The Ton and Tol systems are sophisticated molecular machineries essential for virulence and survival of Gram-negative bacteria. Both systems rely on the proton gradient at the inner membrane to produce force and movement that are transmitted to target proteins associated with the outer membrane. Ton is involved in the uptake of essential nutrients such as siderophore-iron, vitamin B12 and carbohydrates, while Tol maintains outer membrane integrity and plays an active role in cell division. We have solved the high-resolution structures of the E. coli TonB-ExbB-ExbD and TolA-TolQ-TolR complexes, revealing the inner membrane embedded engine parts of the Ton and Tol systems, and showing how TonB and TolA interact with the ExbBD and TolQR subcomplexes.

To stabilize TonB-ExbBD, DDM was replaced with amphipol PMAL-C12 after the first IMAC affinity step, and the remaining purification was performed in the absence of detergent. The stoichiometry of the complex is one TonB subunit, five ExbB and two ExbD. The structure is similar to the reported 3.3 Å resolution structure of ExbBD in MSP1D1 nanodiscs, with the addition of a TM helix of one TonB bound to ExbB chain C (chain IDs according to PDB 6TYI9). The TonB TM is a 35 Å long α-helix, tilted about 15° from the perpendicular axis of the membrane, and interacts with the ExbBC α−1 helix and α−2 TM. Most of the contacts between TonB and ExbBC are located within a region close to the cytoplasm. In this region, the highly conserved TonB residues Ser16 and His20 interact with the ExbB highly conserved Trp38 and Ser34. The cryo-EM map also shows elongated densities in the membrane region at the interface between adjacent ExbB subunits. These densities were attributed to lipids that copurified with the TonB-ExbBD complex. The 2.8 Å resolution consensus structure thus corresponds to a mixed population of TonB-ExbBD, aligned on the TonB subunit, but with ExbBD in three different orientations along the pseudo-5-fold axis. For the remainder of this report, the designation TonB-ExbBD will refer to the consensus 2.8 Å resolution structure with TonB bound to ExbB chain C.

>MGNNLMQTDLSVWGMYQHADIVVKCVMIGLILASVVTWAIFFSKSVEFFNQKRRLKREQQLLAEARSLNQANDIAADFGSKSLSLHLLNEAQNELELSEGSDDNEGIKERTSFRLERRVAAVGRQMGRGNGYLATIGAISPFVGLFGTVWGIMNSFIGIAQTQTTNLAVVAPGIAEALLATAIGLVAAIPAVVIYNVFARQIGGFKAMLGDVAAQVLLLQSRDLDLEASAAAHPVRVAQKLRAG[5x];> MTLDLPRRFPWPTLLSVCIHGAVVAGLLYTSVHQVIELPAPAQPISVTMVTPADLEPPQAVQPPPEPVVEPEPEPEPIPEPPKEAPVVIEKPKPKPKPKPKPVKKVQEQPKRDVKPVESRPASPFENTAPARLTSSTATAATSKPVTSVASGPRALSRNQPQYPARAQALRIEGQVKVKFDVTPDGRVDNVQILSAKPANMFEREVKNAMRRWRYEPGKPGSGIVVNILFKINGTTEIQGGGSENLYFQGGSAWSHPQFEK;>[2x]MAMHLNENLDDNGEMHDINVTPFIDVMLVLLIIFMVAAPLATVDVKVNLPASTSTPQPRPEKPVYLSVKADNSMFIGNDPVTDETMITALNALTEGKKDTTIFFRADKTVDYETLMKVMDTLHQAGYLKIGLVGEETAKAKENLYFQGNAGSGHHHHHHHHHH>[2x]MKQYLELMQKVLDEGTQKNDATGTGTLSIFGHQMRFNLQDGFPLVTTKRCHLRSIIHELLWFLQGDTNIAYLHENNVTIWDEWADENGDLGPVYGKQWRAWPTPDGAHIDQITTVLNQLKNDPDSRRIIVSAWNVGELDKMAL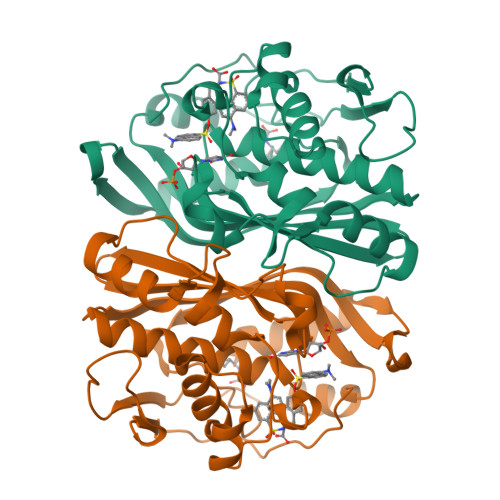APCHAFFQFYVADGKLSCQLYQRSCDVFLGLPFNIASYALLVHMMAQQCDLEVGDFVWTGGDTHLYSNHMDQTHLQLSREPRPLPKLIIKRKPESIFDYRFEDFEIEGYDPHPGIKAPVAI>GSHMVKVCLFVADGTDEIEFSAPWGIFKRAEIPIDSVYVGENKDRLVKMSRDVEMYANRSYKEIPSADDFAKQYDIAIIPGGGLGAKTLSTTPFVQQVVKEFYKKPNKWIGMICAGVLTAKTSGLPNKQITGHPSVRGQLEEGGYKYLDQPVVLEENLITSQGPGTAMLFGLKLLEQVASKDKYNAVYKSLSM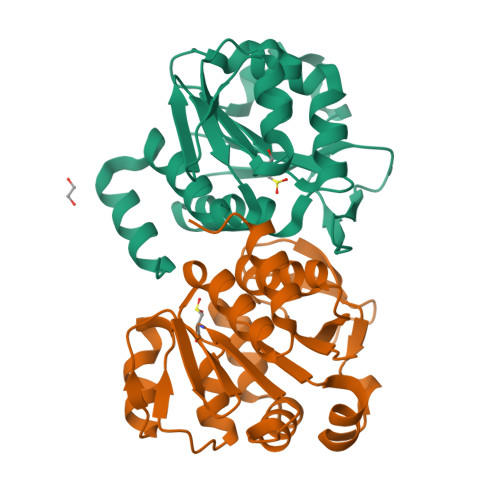P[4x]>[2x]MAHHHHHH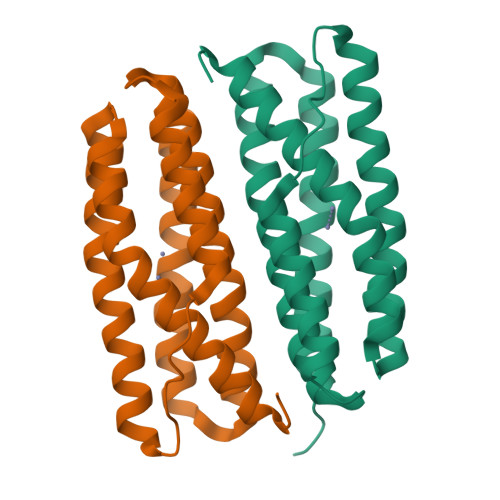MNMKSIEDVFIHLLSDTYSAEKQLTRGLAKLARAASSEKLSAAFNAHLEETQGQIERIDQIIEQESNLKIKRMKCVAMEGLIEEANEVVESTEKNEVRDAALIAAAQKVEHYEIASYGTLVTLAEQLGYKKAAKLLAETLEEEKQTDVKLTDLAVGNINMKAEK>PPAIPGIPGIPGT[6x];>[6x]APDGKKGEAGRPG;>[6x]GIPGMPGLPG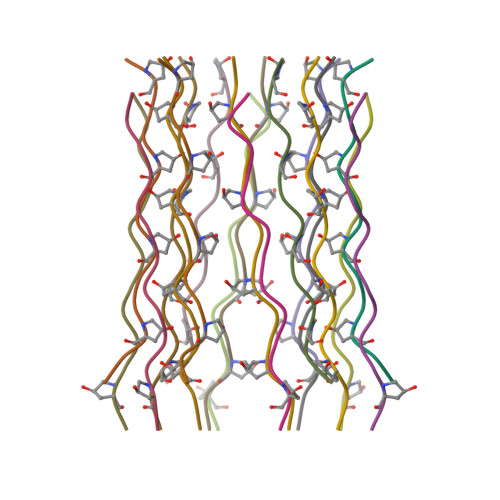APGK> TRDQNGTWEMESNENFEGYMKALDIDFATRKIAVRLTFTLVIDQDGDNFKCKATSTFLNYDVDFTVGVEFDEYTKSLDNRHVKALVTWEGDVLVCVQKGEKENRGWKKWIEGDKLYLELTCGDQVCRQV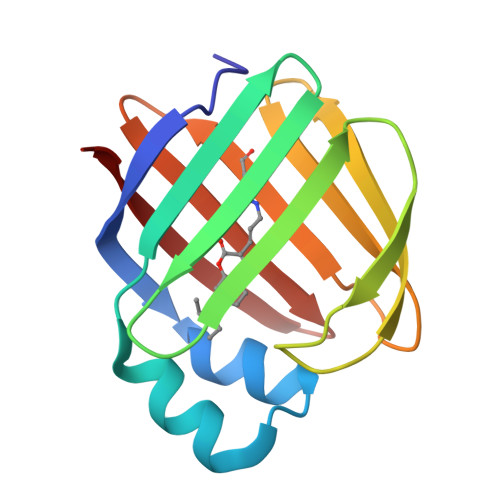FKKK BMP-9 and BMP-10 are TGF-β family signaling ligands naturally secreted into blood. They act on endothelial cells and are required for proper development and maintenance of the vasculature. BMP-9 and −10 are synthesized as pro-proteins and processed by furin to release growth factors comprised of two cystine-knotted protomers that can covalently homo- or hetero-dimerize via a single cysteine in the dimer interface. Unlike other ligands of the TGF-β family, BMP-9 and −10 are secreted as a mixture of disulfide-linked dimers and monomers, in which the interchain cysteine (Cys-392) remains either paired or unpaired.

Hence, purified BMP-9 disulfide-linked dimers were crystallized under neutral pH conditions similar to those used for the cysteinylated monomers. The first fraction of this single crystal analysis had too much free cysteine to model the disulfide-bonded conformation, so datasets from nine crystals of BMP-9 disulfide-linked dimer were split into 8, 16, 32, or 64 parts, and the first fraction from each were combined. The interchain disulfide remains unbroken in the first fraction of the 32 and 64 splits, but is broken and the cysteines are free in the last fraction of all splits. To model the intact interchain disulfide, we inspected the first fraction of the 32 and 64 splits. In the first fraction of the 64 split, automated fit functions still placed the sulfurs beyond disulfide bonding distance, but a manual fit to the omit-map density produces a perfect syn-periplanar (0°) χ3 dihedral angle Cβ-S-S′-Cβ′ with full occupancy. While the observed χ1 dihedral angle of Cys-392 is both an uncommon and high energy conformation, the χ3 dihedral angle (Cβ-S-S′-Cβ′) of the Cys-392-Cys-392’ disulfide is an extreme outlier as the χ3 adopts a syn-periplanar conformation placing the Cβ atoms directly across from each other in the same plane. The intrachain cystines have no outlier dihedral angles and all disulfide bond distances, both inter and intrachain, were acceptable for this resolution. The interchain cystine of BMP-9 has one of the highest energy conformations possible,, yet this is the dominant conformation prior to radiation damage. This is surprising, unless no lower energy conformations are accessible. Analysis of the BMP-9 disulfide-linked dimer structure revealed a highly strained syn-periplanar interchain cystine prior to radiation damage, and an unstrained free cysteine after irradiation.

> SSGAGSHCQKTSLRVNFEDIGWDSWIIAPKEYEAYECKGGCFFPLADDVTPTKHAIVQTLVHLKFPTKVGKACCVPTKLSPISVLYKDDMGVPTLKYHYEGMSVAECGCR>MSVIKPEMKIKLRMEGAVNGHKFVIEGEGIGKPYEGTQTLDLTVKEGAPLPFSYDILTPAFQYGNRAFTKYPKDIPDYFKQAFPEGYSWERSMTYEDQGICIATSDITMEGDCFFYKIRFDGTNFPPNGPVMQKKTLKWEPSTEKMYVRDGVLKGDVNMALLLEGGGHYRCDFKTTYKAKKDVRLPDAHEVDQRIEILSHDKDYNKVRLYEHAEARYSMLPSQAKASGKPIPNPLLGLDSTHHHHHH[4x]

eCGP123 is a bright green FP engineered for extreme stability, and was developed using a two-step process. Phanta was isolated by expression screening of a library targeting amino acid positions 62/63/65/69 and 191/192/193 in the bright green fluorescent protein eCGP123. Phanta contains the substitutions Gln62Met, Thr69Val and His193Gln. The protomers in each protein are typical of the GFP-superfamily and consist of an 11-stranded β-barrel (or β-can) with two small helices forming interconnecting loops protecting the chromophore from bulk solvent.

The absorbance spectrum of eCGP123T69V showed a major absorbing species at 506 nm whilst eCGP123H193Q contained significant amounts of a 387 nm species in addition to the 506 nm species. In the case of eCGP123H193Q titration above pH 8 did not diminish the amount of the protonated form, suggesting that two distinct populations of the chromophore exist, only one of which can be titrated for pH. The results show that under violet light illumination recovery of the ON state for CGP123H193Q driven was minor, whereas thermally induced recovery of the ON state (no illumination) was near complete after 35 mins incubation at 25°C. The conversion OFF to ON rates for Phanta, eCGP123, eCGP123H193Q and eCGP123T69V were determined and are similar. These results suggest that photoswitching of eCGP123H193Q into the ON state is inefficient. The spectral data obtained for eCGP123H193Q suggest the possibility that both the protonated and anionic chromophore are present in the structure but only a single chromophore species appears to be represented in the structural data. However, electron density corresponding to the 4-hyroxybenzyl ring in protomers of both the weakly fluorescent eCGP123H193Q (ΦF, 0.004) and strongly fluorescent eCGP123T69V (ΦF, 0.32) is well defined, indicating a rigid chromophore, and suggesting that a mobile chromophore is not responsible for poor fluorescence emission of eCGP123H193Q. In Phanta and eCGP123H193Q the imidazole ring of His193 is substituted by the polar side chain of a glutamine leaving the chromophore with a reduced number of stabilising interactions. In Phanta and eCGP123H193Q, Glu215 no longer interacts with the side chain of Gln193 that replaces the histidine at position 193. Instead a hydrogen bond is formed between the Nδ1 of Gln193 and the Oγ of Ser142, which in turn forms a hydrogen bond with Oη of the chromophore. In eCGP123H193Q contact between Glu144 and Arg66 is maintained through a water-mediated (H2O783) hydrogen bond. Collectively these data suggest that the very low fluorescence efficiency of Phanta and eCGP123H193Q is a result of removing the stabilising effects of π-π interactions between His193 and the chromophore in the excited state, together with alterations to the scaffold extending around the chromophore.>[2x]GSMDSDEGYNYEFDEDEECSEEDSGAEEEEDEDDDEPDDDTLDLGEVELVEPGLGVGGERDGLLCGETGGGGGSALGPGGGGGGGGGGGGGGPGHEQEEDYRYEVLTAEQILQHMVECIREVNEVIQNPATITRILLSHFNWDKEKLMERYFDGNLEKLFAECHVINPSKKSRTRQMNTRSSAQDMPCQICYLNYPNSYFTGLECGHKFCMQCWSEYLTTKIMEEGMGQTISCPAHGCDILVDDNTVMRLITDSKVKLKYQHLI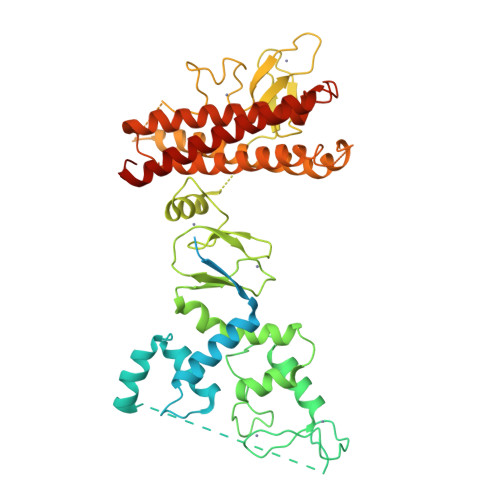TNSFVECNRLLKWCPAPDCHHVVKVQYPDAKPVRCKCGRQFCFNCGENWHDPVKCKWLKKWIKKCDDDSETSNWIAANTKECPKCHVTIEKDGGCNHMVCRNQNCKAEFCWVCLGPWEPHGSAWYNCNRYNEDDAKAARDAQERSRAALQRYLFYCNRYMNHMQSLRFEHKLYAQVKQKMEEMQQHNMSWIEVQFLKKAVDVLCQCRATLMYTYVFAFYLKKNNQSIIFENNQADLENATEVLSGYLERDISQDSLQDIKQKVQDKYRYCESRRRVLLQHVHEGYEKDLWEYIED> MKLPLLLALLFGAVSALHLRSETSTFETPLGAKTLPEDEETPEQEMEETPCRELEEEEEWGSGSEDASKKDGAVESISVPDMVDKNLTCPEEEDTVKVVGIPGCQTCRYLLV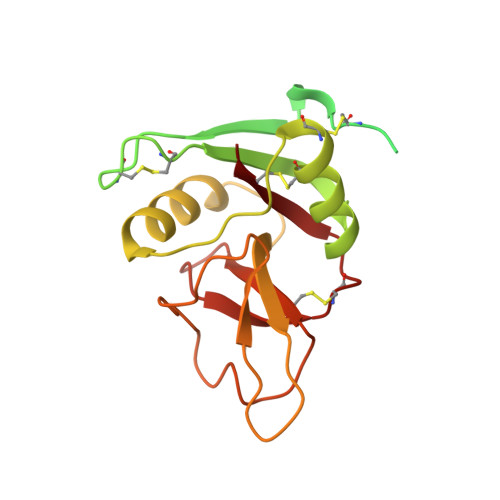RSLQTFSQAWFTCRRCYRGNLVSIHNFNINYRIQCSVSALNQGQVWIGGRITGSGRCRRFQWVDGSRWNFAYWAAHQPWSRGGHCVALCTRGGHWRRAHCLRRLPFICSY(8~{R})-~{N}2-methyl-8-prop-1-ynyl-7,8-dihydro-3~{H}-imidazo[4,5-g]quinazoline-2,6-diamine 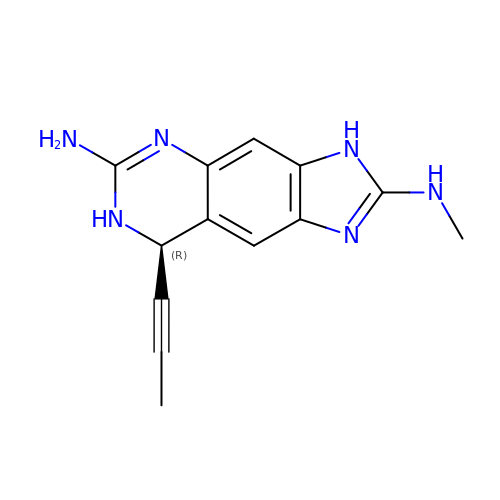| C13 H14 N6 | BBZKTHUVWQCRHC-MRVPVSSYSA-N> MGGHHHHHHGLEVLFQGPRTVKRANGGELKTGYLSIVMDPDELPLDEHCERLPYDASKWEFPRDRLKLGKPLGRGAFGQVIEADAFGIDKTATCRT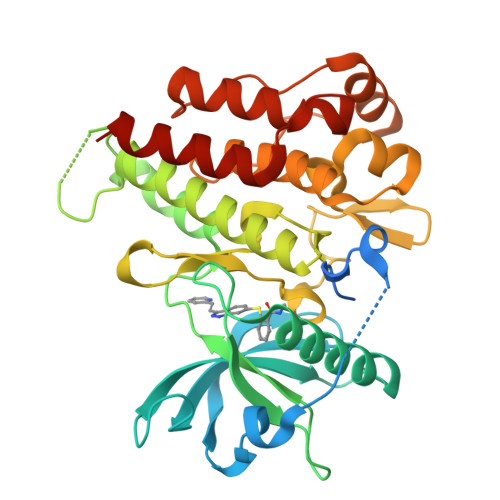VAVKMLKEGATHSEHRALMSELKILIHIGHHLNVVNLLGACTKPGGPLMVIVEFCKFGNLSTYLRSKRNEFVPYKVAPEDLYKDFLTLEHLICYSFQVAKGMEFLASRKCIHRDLAARNILLSEKNVVKICDFGLARDIYKDPDYVRKGDARLPLKWMAPETIFDRVYTIQSDVWSFGVLLWEIFSLGASPYPGVKIDEEFCRRLKEGTRMRAPDYTTPEMYQTMLDCWHGEPSQRPTFSELVEHLGNLLQANAQQD> MKESVRFLTDFGEISDAISDLLTSSPNFNVISAIGPQGAGKSTLLSMLAGNNSRQMYREYVFRPVSREANEQSRHQTIQIDIYIVNHQIFLDCQPMYSFSIMEGLPKVRGGRFDDSTAMSDTLRLTAFLLYVSHTVLVVSETHYDKVIIDTLRVAEQIRPYLAIFRPKLAIDRKTNLVFIKTKASSIDLAPTVIREREELLRLSFQDS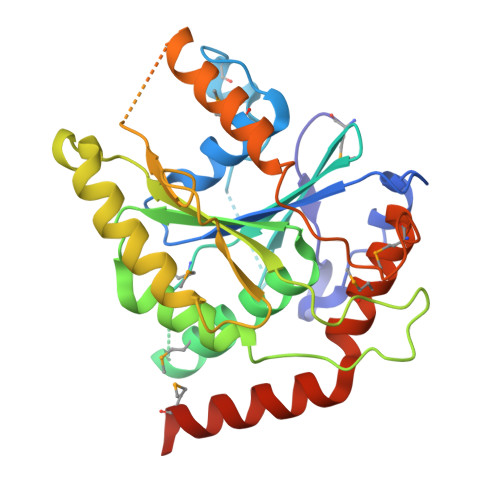RWLKVSQEPFKTLIVLEEIRVRREHLFEEGDEPDEAASLNEFDEQIAELREELQKNREDFTVETAAMDEKKWLDMCREVIRDKTLHKTLKEYQRAMTDGVRTHFDNGFH> PTKPSEGPAKVEEEAAPSIFDEPLERVKN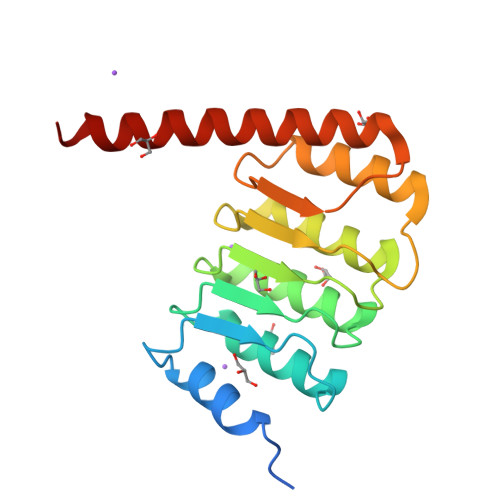NDPEMTEVNVNNSDCITNEILVRFTEALEFNTVVKLFALANTRADDHVAFAIAIMLKANKTITSLNLDSNHITGKGILAIFRALLQNNTLTELRFHNQRHICGGKTEMEIAKLLKENTTLLKLGYHFELAGPRMTVTNLLSRNMDKQRQKRLQEQRQAQ>EFVIEKSLNRIKKFWKEAQYEVIEHSSGLKLVREWDVLEQACKEDLEELVSMKASNYYKIFEQDCLDLESKLTKLSEIQVNWVEVQFYWLDLYGILGENLDIQNFLPLETSKFKSLTSEYKMITTRAFQLDTTIEVIHIPNFDTTLKLTIDSLKMIKSSLSTFLERQRRQFPRFYFLGNDDLLKIIGSGKHHDQVSKFMKKMFGSIESIIFFEDFITGVRSVEGEVLNLNEKIELKDSIQAQEWLNILDTEIKLSVFTQFRDCLGQLKDGTDIEVVVSKYIFQAILLSAQVMWTELVEKCLQTNEFSKYWKEVDMKIKGLLDKLNKSSDNVKKKIEALLVEYLHFNNVIGQLKNCSTKEEARLLWAKVQKFYQKNDTLDDLNSVFISQSGYLLQYKFEYIGIPERLIYTPLLLIGFATLTDSLHQKYGGCFFGPAGTGKTETVKAFGQNLGRVVVVFNCDDSFDYQVLSRLLVGITQIGAWGCFDEFNRLDEKVLSAVSANIQQIQNGLQVGKSHITLLEEETPLSPHTAVFITLNPGYNGRSELPENLKKSFREFSMKSPQSGTIAEMILQIMGFEDSKSLASKIVHFLELLSSKCSSMNHYHFGLRTLKGVLRNCSPLISEFGEGEKTVVESLKRVILPSLGDTDELVFKDELSKIFDSAGTPLNSKAIVQCLKDAGQRSGFSMSEEFLKKCMQFYYMQKTQQALILVGKAGCGKTATWKTVIDAMAIFDGHANVVYVIDTKVLTKESLYGSMLKATLEWRDGLFTSILRRVNDDITGTFKNSRIWVVFDSDLDPEYVEAMNSVLDDNKILTLPNGERLPIPPNFRILFETDNLDHTTPATITRCGLLWFSTDVCSISSKIDHLLNKSYEALDNKLSMFELDKLKDLISDSFDMASLTNIFTCSNDLVHILGVRTFNKLETAVQLAVHLISSYRQWFQNLDDKSLKDVITLLIKRSLLYALAGDSTGESQRAFIQTINTYFGHDSQELSDYSTIVIANDKLSFSSFCSEIPSVSLEAHEVMRPDIVIPTIDTIKHEKIFYDLLNSKRGIILCGPPGSGKTMIMNNALRNSSLYDVVGINFSKDTTTEHILSALHRHTNYVTTSKGLTLLPKSDIKNLVLFCDEINLPKLDKYGSQNVVLFLRQLMEKQGFWKTPENKWVTIERIHIVGACNPPTDPGRIPMSERFTRHAAILYLGYPSGKSLSQIYEIYYKAIFKLVPEFRSYTEPFARASVHLYNECKARYSTGLQSHYLFSPRELTRLVRGVYTAINTGPRQTLRSLIRLWAYEAWRIFADRLVGVKEKNSFEQLLYETVDKYLPNQDLGNISSTSLLFSGLLSLDFKEVNKTDLVNFIEERFKTFCDEELEVPMVIHESMVDHILRIDRALKQVQGHMMLIGASRTGKTILTRFVAWLNGLKIVQPKIHRHSNLSDFDMILKKAISDCSLKESRTCLIIDESNILETAFLERMNTLLANADIPDLFQGEEYDKLLNNLRNKTRSLGLLLDTEQELYDWFVGEIAKNLHVVFTICDPTNNKSSAMISSPALFNRCIINWMGDWDTKTMSQVANNMVDVVPMEFTDFIVPEVNKELVFTEPIQTIRDAVVNILIHFDRNFYQKMKVGVNPRSPGYFIDGLRALVKLVTAKYQDLQENQRFVNVGLEKLNESVLKVNELNKTLPKAPPEEKEASISLVKSLTFEKERWLNTTKQFSKTSQELIGNCIISSIYETYFGHLNERERGDMLVILKRLLGKFAVKYDVNYRFIDYLVTLDEKMKWLECGLDKNDYFLENMSIVMNSQDAVPFLLDPSSHMITVISNYYGNKTVLLSFLEEGFVKRLENAVRFGSVVIIQDGEFFDPIISRLISREFNHAGNRVTVEIGDHEVDVSGDFKLFIHSCDPSGDIPIFLRSRVRLVHFVTNKESIETRIFDITLTEENAEMQRKREDLIKLNTEYRLKLKNLEKRLLEELNNSQGNMLENDELMVTLNNLKKEAMNIEKKLSESEEFFPQFDNLVEEYSIIGKHSVKIFSMLEKFGQFHWFYGISIGQFLSCFKRVFIKKSRETRAARTRVDEILWLLYQEVYCQFSTALDKKFKMIMAMTMFCLYKFDIESEQYKEAVLTMIGVLSESSDGVPKLTVDTNDDLRYLWDYVTTKSYISALNWFKNEFFVDEWNIADVVANSENNYFTMASERDVDGTFKLIELAKASKESLKIIPLGSIENLNYAQEEISKSKIEGGWILLQNIQMSLSWVKTYLHKHVEETKAAEEHEKFKMFMTCHLTGDKLPAPLLQRTDRVVYEDIPGILDTVKDLWGSQFFTGKISGVWSVYCTFLLSWFHALITARTRLVPHGFSKKYYFNDCDFQFASVYLENVLATNSTNNIPWAQVRDHIATIVYGGKIDEEKDLEVVAKLCAHVFCGSDNLQIVPGVRIPQPLLQQSEEEERARLTAILSNTIEPADSLSSWLQLPRESILDYERLQAKEVASSTEQLLQEM[2x];>SPILGYWKIKGLVQPTRLLLEYLEEKYEEHLYERDEGDKWRNKKFELGLEFPNLPYYIDGDVKLTQSMAIIRYIADKHNMLGGCPKERAEI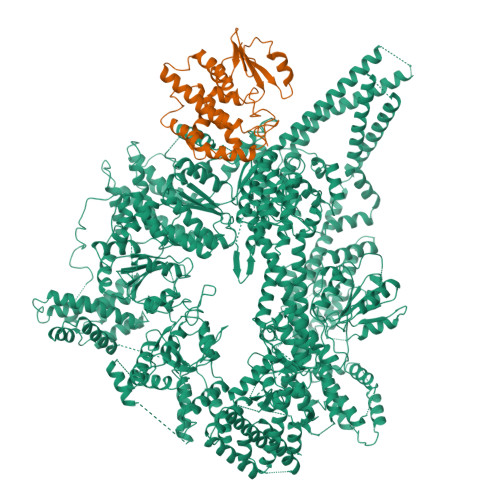SMLEGAVLDIRYGVSRIAYSKDFETLKVDFLSKLPEMLKMFEDRLCHKTYLNGDHVTHPDFMLYDALDVVLYMDPMCLDAFPKLVCFKKRIEAIPQIDKYLKSSKYIAWPLQGWQATFGGGDHPPKSD[2x]> MAVHQIGEGGLVMYWVTFGLMAFSALAFAVMTFTRPLNKRSHGYITLAIVTIAAIAYYAMAASGGKALVSNPDGNLRDIYYARYIDWFFTTPLLLLDIILLTGIPIGVTLWIVLADVAMIMLGLFGALSTNSYRWGYYGVSCAFFFVVLWGLFFPGAKGARARGGQVPGLYFGLAGY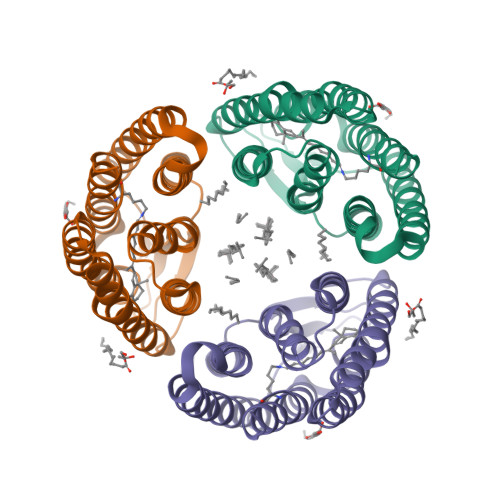LALLWFGYPIVWGLAEGSDYISVTAEAASYAGLDIAAKVVFGWAVMLSHPLIAHHHHHH>MAHHHHHHMSEAKLFSPLKVGAVTVPNRVFMAPLTRLRSIEPGDIPTPLMGEYYRQRASSGLIITEATQISAQAKGYAGAPGLHSPEQIAAWQKITAGVHAENGHIAVQLWHTGRISHSSLQPGGAAPVAPSALSAGTRTSLRDENGHAIRVDTSMPRALETAEIPGIVNDFRQAVGNARDAGFDLVELHSAHGYLLHQFLSPSANQRTDQYGGSVENRARLVLEVVDAVSQEWSAERIGIRVSPIGSFQNVDNGPNEEEDALYLISELAKRGIAYLHMSEPDWAGGKPYSEAFRQKVRDRFPGVIIGAGAYTVE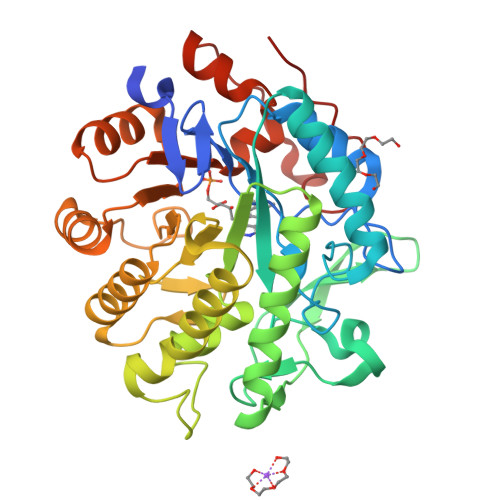KANDLINKGLIDAVAFGRDYIANPDLVARLQKKAPLNPQRPESFYGGGAEGYTDYPTL[6x]>MKHLGQTRSALHGSHAVITPETFVRTALAEWPGSAIVLHIAPVVGLGARFVQFTAEMPAGAQATESVYQRFAFVLSGEVDVAVGGETRTLREYDYVYLPAGEKHMLTAKTDARVSVFEKPYQTVEGVQAPGVYWGNERENPGYPFEGDDHLIARKLLPDEPAFDFMVSTMSFAPGASLPYAEVHYMEHGLLML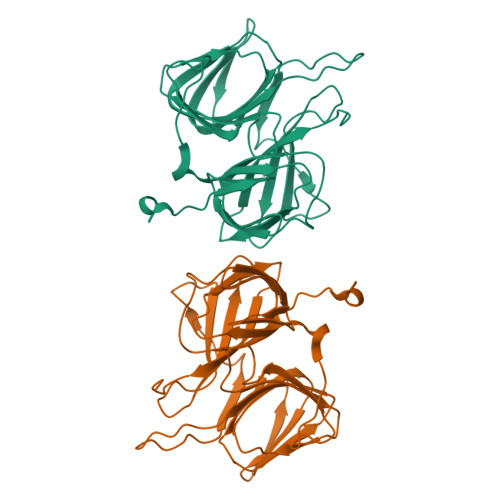EGEGLYKLEENYYPVTAGDIIWMGAHCPQWYGALGRNWSKYLLYKDMNRHPLG[2x]> KQMVLQQALPMTLKGLDKASELATLTPEGLAREHSRLASGDGALRSLSTALAGIRAGSQVEESRIQAGRLLERSIGGIALQQWGTTGGAASQLVLDA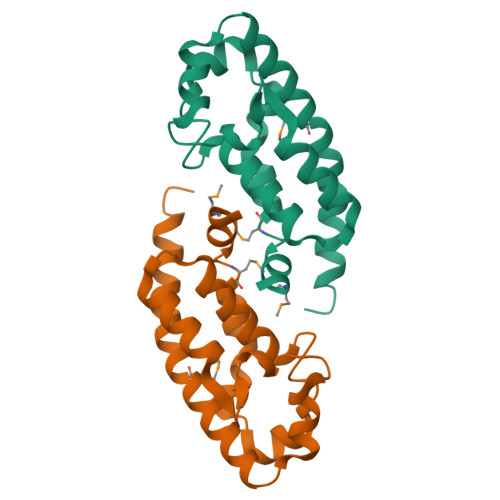SPELRREITDQLHQVMSEVALLRQAVESEVSRVSADY>[2x]MALRVGIVYGTRPEAIKLAPLVLALDADPGFEPVIITTGQHRDMLDEINELFGLRPRHNLDIMRPGQRLSAMASRIVGELGDPLLDELVDVAVVQGDTSTAFAAAYAAACERIPVAHLEAGLRTGDRFEPFPEEINRRLITQLADLHFAPTADAAGNLLAEGVRSDDVYVTGNTVIDAMHLVLDRPGDSANRELDAFTEGRQTVLLTMHRRES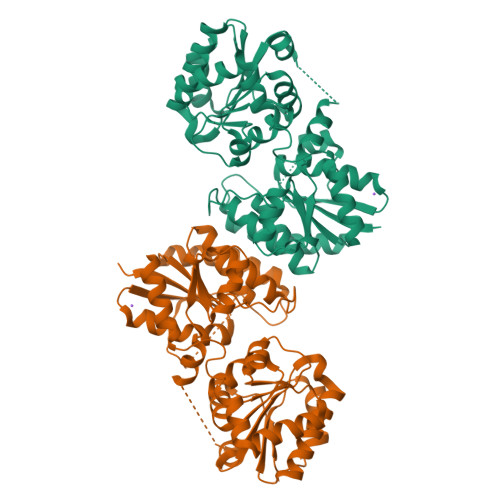WGIPMGRVAAAVAELCRSRPTLRFVIPLHPNPEVRRVFRSHLSSLTQVLLCEPLRYSEFIRLMHRAVLVLTDSGGVQEEAPTLGKPVLVLRDRTERPEGIAAGCARLVGTDPALIVKEVGRLLDDPEAYEAMRRPGIVCYGEGDAAARCLEALRERWLSSPDASAGLRTYR>[3x]MEGNTILKIVLICTILAGLFGQVVPVYAENTTYQTPTGIYYEVRGDTIYMINVTSGEETPIHLFGVNWFGFETPNHVVHGLWKRNWEDMLLQIKSLGFNAIRLPFCTESVKPGTQPIGIDYSKNPDLRGLDSLQIMEKIIKKAGDLGIFVLLDYHRIGCTHI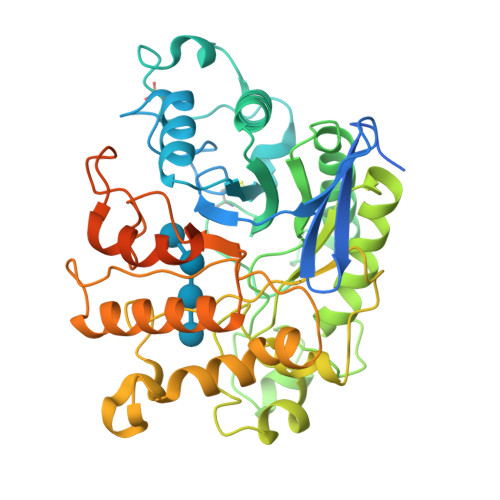EPLWYTEDFSEEDFINTWIEVAKRFGKYWNVIGADLKNEPHSVTSPPAAYTDGTGATWGMGNPATDWNLAAERIGKAILKVAPHWLIFVEGTQFTNPKTDSSYKWGYNAWWGGNLMAVKDYPVNLPRNKLVYSPHVFGPDVYNQPYFGPAKGFPDNLPDIWYHHFGYVKLELGYSVVIGEFGGKYGHGGDPRDVIWQNKLVDWMIENKFCDFFYWSWNPDSGDTGGILQDDWTTIWEDKYNNLKRLMDSCSKSSSSTQSVIRSTTPTKSNTSKKICGPAILIILAVFSLLLRRAPR>[2x]APLAPPLAEDRSYRTWRVEDYVEAWERYHGREMTEDERENLARGCIGVTVVNLNREDLSNPPLNLSFGSLRTAEAVQAALNKIVDTHPSPAQYEAAVAKDPILKRLKNVVKALPSWIDSAKLKASIFSKRFYSWQNPDWSEERAHTTYRPDRETDQVDMSTYRYRARPGYVNFDYGWFDQDTNTWWHANHEEPRMVVYQSTLRHYSRPLQDFDEQVFTVAFAKKD

Transglutaminases catalyze the formation of a stable isopeptide bond between an acyl group (e.g. a glutamine side chain) and an alkyl amine (e.g. a lysine side chain). In contrast to mammalian transglutaminases, bacterial enzymes do not require cofactors, such as Ca2+ or GTP, and function over a broad range of pH, buffers, and temperatures. The K. albida gene product is significantly smaller than MTG, amounting to a calculated molecular mass of 30.1 kDa and a molecular mass of 26.4 kDa in the active form.

To gain further insight into how the small KalbTG sequence can fold into such an efficient MTG and whether the substrate specificity as determined by the peptide array can be explained, we determined the crystal structure of KalbTG to a resolution of 1.9 Å. Superposition of KalbTG with its next closest homolog, the MTG from S. mobaraensis, shows a similar disc-shaped core structure (root mean square deviation of 1.5 Å) of a central β-sheet with flanking α-helices and a surface depression forming the active site cleft. However, KalbTG is more compact, having much shorter surface loops. The catalytic Cys-Asp-His triad of KalbTG is located at the bottom of the active site groove. The groove is wide enough to be covered by a kinked helical propeptide in the unprocessed enzyme, similar to what has been observed with the S. mobaraensis MTG zymogen, indicating that a similar zymogenic mechanism may be present in KalbTG. Strong difference electron density extending from Cγ of the catalytic Cys-82 showed that this residue is modified by a thiol-reactive compound, the origin of which is unknown. The electron density allows tracing of four atoms, and these were tentatively modeled as a β-mercaptoethanol disulfide adduct of Cys-82. As in all other transglutaminase structures, the catalytic Cys-82 in KalbTG is located at the N terminus of an α-helix, which reduces its pKa and increases its nucleophilicity for attack on the substrate glutamine. Of note, the catalytic Cys-82 in KalbTG is embedded 1.7 Å deeper in the active cleft than its S. mobaraensis MTG counterpart, raising the question of how the Gln side chain of the substrate peptide might reach it. However, these are difficult to distinguish from water in electron density maps, and no NH4+ has been identified in the KalbTG structure based on geometric criteria (four hydrogen bond acceptors in a tetrahedral geometry).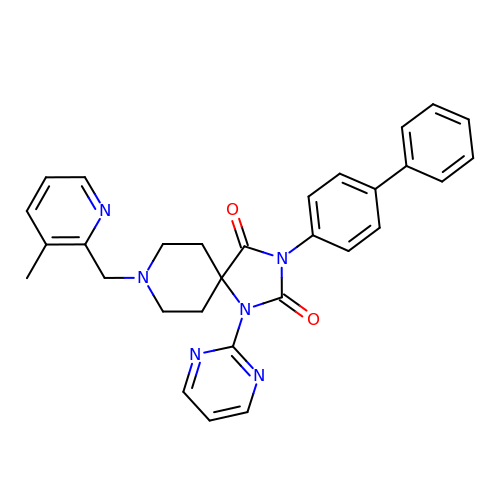8-[(3-methylpyridin-2-yl)methyl]-3-(4-phenylphenyl)-1-pyrimidin-2-yl-1,3,8-triazaspiro[4.5]decane-2,4-dione | C30 H28 N6 O2 | FIMHRJKSKVXMEB-UHFFFAOYSA-N The MCM motor of the eukaryotic replicative helicase is loaded as a double hexamer onto DNA by the Origin Recognition Complex (ORC), Cdc6, and Cdt1. ATP binding supports formation of the ORC-Cdc6-Cdt1-MCM (OCCM) helicase-recruitment complex where ORC-Cdc6 and one MCM hexamer form two juxtaposed rings around duplex DNA. MCM is a ring-shaped helicase containing six related AAA+ ATPase polypeptides featuring bipartite active sites with catalytic residues contributed by neighbouring subunits. Biochemical studies established that ATP hydrolysis by MCM, but not ORC or Cdc6, are essential to complete helicase loading.

To further understand the role of ATP hydrolysis in OCCM-to-SH transition, we assembled a DH loading reaction using MCM-Cdt1 bearing the Mcm5RA variant. 3D classification identified two distinct states of a complex containing ORC-Cdt1-MCM but lacking Cdc6 (OC1MMcm5RA). While all ORC subunits are visible, the two states differ in the configuration of Orc1. In conformer 1, solved to 3.7 Å resolution both the C-terminal WHD domain of Orc1 can be observed as well as the ATPase domain (though local resolution of the latter is lower). Orc1 ATPase is engaged in AAA+ interaction with the neighbouring Orc4 subunit, with ATP bound at the interface. In turn, for OC1MMcm5RA we observe two states, co-existing after Cdc6 release. In one state, the full Orc1 subunit is visible, and its ATPase domain is flexible yet still engaged to the neighbouring Orc4 subunit. Compared to the OCCMMcm2RA, which contains a three-subunit ATPase spiral, the Mcm5 subunit engages Mcm2 in OC1MMcm5RA, capping the N-terminal end of a four-subunit spiral. Nucleotide (ADP, according to the cryo-EM density) can be observed bound to each of the Mcm4-6-2-5 subunits forming the ATPase spiral, but not to the Mcm3 and Mcm7 subunits. Mcm5 establishes new contacts with DNA downstream of the Mcm2 DNA binding sites and away from ORC.

> MSDNRRRRREEDDSDSENELPPSSPQQHFRGGMNPVSSPIGSPDMINPEGDDNEVDDVPDIDEVEEQMNEVDLMDDNMYEDYAADHNRDRYDPDQVDDREQQELSLSERRRIDAQLNERDRLLRNVAYIDDEDEEQEGAAQLDEMGLPVQRRRRRRQYEDLENSDDDLLSDMDIDPLREELTLESLSNVKANSYSEWITQPNVSRTIARELKSFLLEYTDETGRSVYGARIRTLGEMNSESLEVNYRHLAESKAILALFLAKCPEEMLKIFDLVAMEATELHYPDYARIHSEIHVRISDFPTIYSLRELRESNLSSLVRVTGVVTRRTGVFPQLKYVKFNCLKCGSILGPFFQDSNEEIRISFCTNCKSKGPFRVNGEKTVYRNYQRVTLQEAPGTVPPGRLPRHREVILLADLVDVSKPGEEVEVTGIYKNNYDGNLNAKNGFPVFATIIEANSIKRREGNTANEGEEGLDVFSWTEEEEREFRKISRDRGIIDKIISSMAPSIYGHRDIKTAVACSLFGGVPKNVNGKHSIRGDINVLLLGDPGTAKSQILKYVEKTAHRAVFATGQGASAVGLTASVRKDPITKEWTLEGGALVLADKGVCLIDEFDKMNDQDRTSIHEAMEQQSISISKAGIVTTLQARCSIIAAANPNGGRYNSTLPLAQNVSLTEPILSRFDILCVVRDLVDEEADERLATFVVDSHVRSHPENDEDREGEELKNNGESAIEQGEDEINEQLNARQRRLQRQRKKEEEISPIPQELLMKYIHYARTKIYPKLHQMDMDKVSRVYADLRRESISTGSFPITVRHLESILRIAESFAKMRLSEFVSSYDLDRAIKVVVDSFVDAQKVSVRRQLRRSFAIYTLGH;> MKRRWKKNFIAVSAANRFKKISSSGALENLYFQGEMEGSTGFDGDATTFFAPDAVFGDRVRRFQEFLDTFTSYRDSVRSIQVYNSNNAANYNDDQDDADERDLLGDDDGDDLEKEKKAASSTSLNILPHRIIISLDDLREFDRSFWSGILVEPAYFIPPAEKALTDLADSMDDVPHPNASAVSSRHPWKLSFKGSFGAHALSPRTLTAQHLNKLVSVEGIVTKTSLVRPKLIRSVHYAAKTGRFHYRDYTDATTTLTTRIPTPAIYPTEDTEGNKLTTEYGYSTFIDHQRITVQEMPEMAPAGQLPRSIDVILDDDLVDKTKPGDRVNVVGVFKSLGAGGMNQSNSNTLIGFKTLILGNTVYPLHARSTGVAARQMLTDFDIRNINKLSKKKDIFDILSQSLAPSIYGHDHIKKAILLMLMGGVEKNLENGSHLRGDINILMVGDPSTAKSQLLRFVLNTASLAIATTGRGSSGVGLTAAVTTDRETGERRLEAGAMVLADRGVVCIDEFDKMTDVDRVAIHEVMEQQTVTIAKAGIHTTLNARCSVIAAANPVFGQYDVNRDPHQNIALPDSLLSRFDLLFVVTDDINEIRDRSISEHVLRTHRYLPPGYLEGEPVRERLNLSLAVGEDADINPEEHSNSGAGVENEGEDDEDHVFEKFNPLLQAGAKLAKNKGNYNGTEIPKLVTIPFLRKYVQYAKERVIPQLTQEAINVIVKNYTDLRNDDNTKKSPITARTLETLIRLATAHAKVRLSKTVNKVDAKVAANLLRFALLGEDIGNDIDEEESEYEEALSKRSPQKSPKKRQRVRQPASNSGSPIKSTPRRSTASSVNATPSSARRILRFQDDEQNAGEDDNDIMSPLPADEEAELQRRLQLGLRVSPRRREHLHAPEEGSSGPLTEVGTPRLPNVSSAGQDDEQQQSVISFDNVEPGTISTGRLSLISGIIARLMQTEIFEEESYPVASLFERINEELPEEEKFSAQEYLAGLKIMSDRNNLMVADDKVWRV;> MSQQSSSPTKEDNNSSSPVVPNPDSVPPQLSSPALFYSSSSSQGDIYGRNNSQNLSQGEGNIRAAIGSSPLNFPSSSQRQNSDVFQSQGRQGRIRSSASASGRSRYHSDLRSDRALPTSSSSLGRNGQNRVHMRRNDIHTSDLSSPRRIVDFDTRSGVNTLDTSSSSAPPSEASEPLRIIWGTNVSIQECTTNFRNFLMSFKYKFRKILDEREEFINNTTDEELYYIKQLNEMRELGTSNLNLDARNLLAYKQTEDLYHQLLNYPQEVISIMDQTIKDCMVSLIVDNNLDYDLDEIETKFYKVRPYNVGSCKGMRELNPNDIDKLINLKGLVLRSTPVIPDMKVAFFKCNVCDHTMAVEIDRGVIQEPARCERIDCNEPNSMSLIHNRCSFADKQVIKLQETPDFVPDGQTPHSISLCVYDELVDSCRAGDRIEVTGTFRSIPIRANSRQRVLKSLYKTYVDVVHVKKVSDKRLDVDTSTIEQELMQNKVDHNEVEEVRQITDQDLAKIREVAAREDLYSLLARSIAPSIYELEDVKKGILLQLFGGTNKTFTKGGRYRGDINILLCGDPSTSKSQILQYVHKITPRGVYTSGKGSSAVGLTAYITRDVDTKQLVLESGALVLSDGGVCCIDEFDKMSDSTRSVLHEVMEQQTISIAKAGIITTLNARSSILASANPIGSRYNPNLPVTENIDLPPPLLSRFDLVYLVLDKVDEKNDRELAKHLTNLYLEDKPEHISQDDVLPVEFLTMYISYAKEHIHPIITEAAKTELVRAYVGMRKMGDDSRSDEKRITATTRQLESMIRLAEAHAKMKLKNVVELEDVQEAVRLIRSAIKDYATDPKTGKIDMNLVQTGKSVIQRKLQEDLSREIMNVLKDQASDSMSFNELIKQINEHSQDRVESSDIQEALSRLQQEDKVIVLGEGVRRSVRLNNRV;> MSFDRPEIYSAPVLQGESPNDDDNTEIIKSFKNFILEFRLDSQFIYRDQLRNNILVKNYSLTVNMEHLIGYNEDIYKKLSDEPSDIIPLFETAITQVAKRISILSRAQSANNNDKDPENTSMDTDSLLLNSLPTFQLILNSNANQIPLRDLDSEHVSKIVRLSGIIISTSVLSSRATYLSIMCRNCRHTTSITINNFNSITGNTVSLPRSCLSTIESESSMANESNIGDESTKKNCGPDPYIIIHESSKFIDQQFLKLQEIPELVPVGEMPRNLTMTCDRYLTNKVIPGTRVTIVGIYSIYNSKNGAGSGRSGGGNGGSGVAIRTPYIKILGIQSDVETSSIWNSVTMFTEEEEEEFLQLSRNPKLYEILTNSIAPSIFGNEDIKKAIVCLLMGGSKKILPDGMRLRGDINVLLLGDPGTAKSQLLKFVEKVSPIAVYTSGKGSSAAGLTASVQRDPMTREFYLEGGAMVLADGGVVCIDEFDKMRDEDRVAIHEAMEQQTISIAKAGITTVLNSRTSVLAAANPIYGRYDDLKSPGDNIDFQTTILSAFDMIFIVKDDHNEERDISIANHVINIHTGNANAMQNQQEENGSEISIEKMKRYITYCRLKCAPRLSPQAAEKLSSNFVTIRKQLLINELESTERSSIPITIRQLEAIIRITESLAKLELSPIAQERHVDEAIRLFQASTMDAASQDPIGGLNQASGTSLSEIRRFEQELKRRLPIGWSTSYQTLRREFVDTHRFSQLALDKALYALEKHETIQLRHQGQNIYRSGV;> MSSPFPADTPSSNRPSNSSPPPSSIGAGFGSSSGLDSQIGSRLHFPSSSQPHVSNSQTGPFVNDSTQFSSQRLQTDGSATNDMEGNEPARSFKSRALNHVKKVDDVTGEKVREAFEQFLEDFSVQSTDTGEVEKVYRAQIEFMKIYDLNTIYIDYQHLSMRENGALAMAISEQYYRFLPFLQKGLRRVVRKYAPELLNTSDSLKRSEGDEGQADEDEQQDDDMNGSSLPRDSGSSAAPGNGTSAMATRSITTSTSPEQTERVFQISFFNLPTVHRIRDIRSEKIGSLLSISGTVTRTSEVRPELYKASFTCDMCRAIVDNVEQSFKYTEPTFCPNPSCENRAFWTLNVTRSRFLDWQKVRIQENANEIPTGSMPRTLDVILRGDSVERAKPGDRCKFTGVEIVVPDVTQLGLPGVKPSSTLDTRGISKTTEGLNSGVTGLRSLGVRDLTYKISFLACHVISIGSNIGASSPDANSNNRETELQMAANLQANNVYQDNERDQEVFLNSLSSDEINELKEMVKDEHIYDKLVRSIAPAVFGHEAVKKGILLQMLGGVHKSTVEGIKLRGDINICVVGDPSTSKSQFLKYVVGFAPRSVYTSGKASSAAGLTAAVVRDEEGGDYTIEAGALMLADNGICCIDEFDKMDISDQVAIHEAMEQQTISIAKAGIHATLNARTSILAAANPVGGRYNRKLSLRGNLNMTAPIMSRFDLFFVILDDCNEKIDTELASHIVDLHMKRDEAIEPPFSAEQLRRYIKYARTFKPILTKEARSYLVEKYKELRKDDAQGFSRSSYRITVRQLESMIRLSEAIARANCVDEITPSFIAEAYDLLRQSIIRVDVDDVEMDEEFDNIESQSHAASGNNDDNDDGTGSGVITSEPPADIEEGQSEATARPGTSEKKKTTVTYDKYVSMMNMIVRKIAEVDREGAEELTAVDIVDWYLLQKENDLGSLAEYWEERRLAFKVIKRLVKDRILMEIHGTRHNLRDLENEENENNKTVYVIHPNCEVLDQLEPQDSS;> MSAALPSIQLPVDYNNLFNEITDFLVTFKQDTLSSDATRNENEDENLDAENIEQHLLEKGPKYMAMLQKVANRELNSVIIDLDDILQYQNEKFLQGTQADDLVSAIQQNANHFTELFCRAIDNNMPLPTKEIDYKDDVLDVILNQRRLRNERMLSDRTNEIRSENLMDTTMDPPSSMNDALREVVEDETELFPPNLTRRYFLYFKPLSQNCARRYRKKAISSKPLSVRQIKGDFLGQLITVRGIITRVSDVKPAVEVIAYTCDQCGYEVFQEVNSRTFTPLSECTSEECSQNQTKGQLFMSTRASKFSAFQECKIQELSQQVPVGHIPRSLNIHVNGTLVRSLSPGDIVDVTGIFLPAPYTGFKALKAGLLTETYLEAQFVRQHKKKFASFSLTSDVEERVMELITSGDVYNRLAKSIAPEIYGNLDVKKALLLLLVGGVDKRVGDGMKIRGDINVCLMGDPGVAKSQLLKAICKISPRGVYTTGKGSSGVGLTAAVMKDPVTDEMILEGGALVLADNGICCIDEFDKMDESDRTAIHEVMEQQTISISKAGINTTLNARTSILAAANPLYGRYNPRLSPLDNINLPAALLSRFDILFLMLDIPSRDDDEKLAEHVTYVHMHNKQPDLDFTPVEPSKMREYIAYAKTKRPVMSEAVNDYVVQAYIRLRQDSKREMDSKFSFGQATPRTLLGIIRLSQALAKLRLADMVDIDDVEEALRLVRVSKESLYQETNKSKEDESPTTKIFTIIKKMLQETGKNTLSYENIVKTVRLRGFTMLQLSNCIQEYSYLNVWHLINEGNTLKFVDDGTMDTDQEDSLVSTPKLAPQTTASANVSAQDSDIDLQDA;> MSGTANSRRKEVLRVPVIDLNRVSDEEQLLPVVRAILLQHDTFLLKNYANKAVLDALLAGLTTKDLPDTSQGFDANFTGTLPLEDDVWLEQYIFDTDPQLRFDRKCRNESLCSIYSRLFKLGLFFAQLCVKSVVSSAELQDCISTSHYATKLTRYFNDNGSTHDGADAGATVLPTGDDFQYLFERDYVTFLPTGVLTIFPCAKAIRYKPSTMATTDNSWVSIDEPDCLLFHTGTLLARWSQGMHTTSPLQIDPRANIVSLTIWPPLTTPISSKGEGTIANHLLEQQIKAFPKVAQQYYPRELSILRLQDAMKFVKELFTVCETVLSLNALSRSTGVPPELHVLLPQISSMMKRKIVQDDILKLLTIWSDAYVVELNSRGELTMNLPKRDNLTTLTNKSRTLAFVERAESWYQQVIASKDEIMTDVPAFKINKRRSSSNSKTVLSSKVQTKSSNANALNNSRYLANSKENFMYKEKMPDSQANLMDRLRERERRSAALLSQRQKRYQQFLAMKMTQVFDILFSLTRGQPYTETYLSSLIVDSLQDSNNPIGTKEASEILAGLQGILPMDISVHQVDGGLKVYRWNSLDKNRFSKLLQIHKSKQQD;> MKRRWKKNFIAVSAANRFKKISSSGALENLYFQGEMAKTLKDLQGWEIITTDEQGNIIDGGQKRLRRRGAKTEHYLKRSSDGIKLGRGDSVVMHNEAAGTYSVYMIQELRLNTLNNVVELWALTYLRWFEVNPLAHYRQFNPDANILNRPLNYYNKLFSETANKNELYLTAELAELQLFNFIRVANVMDGSKWEVLKGNVDPERDFTVRYICEPTGEKFVDINIEDVKAYIKKVEPREAQEYLKDLTLPSKKKEIKRGPQKKDKATQTAQISDAETRATDITDNEDGNEDESSDYESPSDIDVSEDMDSGEISADELEEEEDEEEDEDEEEKEARHTNSPRKRGRKIKLGKDDIDASVQPPPKKRGRKPKDPSKPRQMLLISSCRANNTPVIRKFTKKNVARAKKKYTPFSKRFKSIAAIPDLTSLPEFYGNSSELMASRFENKLKTTQKHQIVETIFSKVKKQLNSSYVKEEILKSANFQDYLPARENEFASIYLSAYSAIESDSATTIYVAGTPGVGKTLTVREVVKELLSSSAQREIPDFLYVEINGLKMVKPTDCYETLWNKVSGERLTWAASMESLEFYFKRVPKNKKKTIVVLLDELDAMVTKSQDIMYNFFNWTTYENAKLIVIAVANTMDLPERQLGNKITSRIGFTRIMFTGYTHEELKNIIDLRLKGLNDSFFYVDTKTGNAILIDAAGNDTTVKQTLPEDVRKVRLRMSADAIEIASRKVASVSGDARRALKVCKRAAEIAEKHYMAKHGYGYDGKTVIEDENEEQIYDDEDKDLIESNKAKDDNDDDDDNDGVQTVHITHVMKALNETLNSHVITFMTRLSFTAKLFIYALLNLMKKNGSQEQELGDIVDEIKLLIEVNGSNKFVMEIAKTLFQQGSDNISEQLRIISWDFVLNQLLDAGILFKQTMKNDRICCVKLNISVEEAKRAMNEDETLRNL;> SPDPALKPKTPSKAPRKRGRPRKIQEELTDRIKKDEKDTISSKKKRKLDKDTSGNVNEESKTSNNKQVMEKTGIKEKREREKIQVATTTYEDNVTPQTDDNFVSNSPEPPEPATPSKKSLTTNHDFTSPLKQIIMNNLKEYKDSTSPGKLTLSRNFTPTPVPKNKKLYQTSETKSASSFLDTFEGYFDQRKIVRTNAKSRHTMSMAPDVTREEFSLVSNFFNENFQKRPRQKLFEIQKKMFPQYWFELTQGFSLLFYGVGSKRNFLEEFAIDYLSPKIAYSQLAYENELQQNKPVNSIPCLILNGYNPSCNYRDVFKEITDLLVPAELTRSETKYWGNHVILQIQKMIDFYKNQPLDIKLILVVHNLDGPSIRKNTFQTMLSFLSVIRQIAIVASTDHIYAPLLWDNMKAQNYNFVFHDISNFEPSTVESTFQDVMKMGKSDTSSGAEGAKYVLQSLTVNSKKMYKLLIETQMQNMGNLSANTGPKRGTQRTGVELKLFNHLCAADFIASNEIALRSMLREFIEHKMANITKNNSGMEIIWVPYTYAELEKLLKTVLNTL;> MSDLNQSKKMNVSEFADAQRSHYTVYPSLPQSNKNDKHIPFVKLLSGKESEVNVEKRWELYHQLHSHFHDQVDHIIDNIEADLKAEISDLLYSETTQKRRCFNTIFLLGSDSTTKIELKDESSRYNVLIELTPKESPNVRMMLRRSMYKLYSAADAEEHPTIKYEDINDEDGDFTEQNNDVSYDLSLVENFKRLFGKDLAMVFNFKDVDSINFNTLDNFIILLKSAFKYDHVKISLIFNINTNLSNIEKNLRQSTIRLLKRNYHKLDVSSNKGFKYGNQIFQSFLDTVDGKLNLSDRFVEFILSKMANNTNHNLQLLTKMLDYSLMSYFFQNAFSVFIDPVNVDFLNDDYLKILSRCPTFMFFVEGLIKQHAPADEILSLLTNKNRGLEEFFVEFLVRENPINGHAKFVARFLEEELNITNFNLIELYHNLLIGKLDSYLDRWSACKEYKDRLHFEPIDTIFQELFTLDNRSGLLTQSIFPSYKSNIEDNLLSWEQVLPSLDKENYDTLSGDLDKIMAPVLGQLFKLYREANMTINIYDFYIAFRETLPKEEILNFIRKDPSNTKLLELAETPDAFDKVALILFMQAIFAFENMGLIKFQSTKSYDLVEKCVWRGI;> MTISEARLSPQVNLLPIKRHSNEEVEETAAILKKRTIDNEKCKDSDPGFGSLQRRLLQQLYGTLPTDEKIIFTYLQDCQQEIDRIIKQSIIQKESHSVILVGPRQSYKTYLLDYELSLLQQSYKEQFITIRLNGFIHSEQTAINGIATQLEQQLQKIHGSEEKIDDTSLETISSGSLTEVFEKILLLLDSTTKTRNEDSGEVDRESITKITVVFIFDEIDTFAGPVRQTLLYNLFDMVEHSRVPVCIFGCTTKLNILEYLEKRVKSRFSQRVIYMPQIQNLDDMVDAVRNLLTVRSEISPWVSQWNETLEKELSDPRSNLNRHIRMNFETFRSLPTLKNSIIPLVATSKNFGSLCTAIKSCSFLDIYNKNQLSNNLTGRLQSLSDLELAILISAARVALRAKDGSFNFNLAYAEYEKMIKAINSRIPTVAPTTNVGTGQSTFSIDNTIKLWLKKDVKNVWENLVQLDFFTEKSAVGLRDNATAAFYASNYQFQGTMIPFDLRSYQMQIILQELRRIIPKSNMYYSWTQL;> MNVTTPEVAFREYQTNCLASYISADPDITPSNLILQGYSGTGKTYTLKKYFNANPNLHAVWLEPVELVSWKPLLQAIARTVQYKLKTLYPNIPTTDYDPLQVEEPFLLVKTLHNIFVQYESLQEKTCLFLILDGFDSLQDLDAALFNKYIKLNELLPKDSKINIKFIYTMLETSFLQRYSTHCIPTVMFPRYNVDEVSTILVMSRCGELMEDSCLRKRIIEEQITDCTDDQFQNVAANFIHLIVQAFHSYTGNDIFALNDLIDFKWPKYVSRITKENIFEPLALYKSAIKLFLSTDDNLSENGQGESAITTNRDDLENSQTYDLSIISKYLLIASYICSYLEPRYDASIFSRKTRIIQGRAAYGRRKKKEVNPRYLQPSLFAIERLLAIFQAIFPIQGKAESGSLSALREESLMKANIEVFQNLSELHTLKLIATTMNKNIDYLSPKVRWKVNVPWEIIKEISESVHFNISDYFSDIHE;> MSMQQVQHCVAEVLRLDPQEKPDWSSGYLKKLTNATSILYNTSLNKVMLKQDEEVARCHICAYIASQKMNEKHMPDLCYYIDSIPLEPKKAKHLMNLFRQSLSNSSPMKQFAWTPSPKKNKRSPVKNGGRFTSSDPKELRNQLFGTPTKVRKSQNNDSFVIPELPPMQTNESPSITRRKLAFEEDEDEDEEEPGNDGLSLKSHSNKSITGTRNVDSDEYENHESDPTSEEEPLGVQESRSGRTKQNKAVGKPQSELKTAKALRKRGRIPNSLLVKKYCKMTTEEIIRLCNDFELPREVAYKIVDEYNINASRLVCPWQLVCGLVLNCTFIVFNERRRKDPRIDHFIVSKMCSLMLTSKVDDVIECVKLVKELIIGEKWFRDLQIRYDDFDGIRYDEIIFRKLGSMLQTTNILVTDDQYNIWKKRIEMDLALTEPL>[4x]MNVTVDQSTLAGATRGIVRGGETLKEHRDRLMAATKATGRYAGLKTLELREREPILYNKLFSRLRAGVVDARETAKKIAASPIVEQEGELCFTLYNAAGDSLLTSTGIIIHVGTMGAAIKYMIENNWEANPGVHDKDIFCNNDSLIGNVHPCDIHTIVPIFWEGELIGWVGGVTHVIDTGAVGPGSMATGQVQRFGDGYSITCRKVGANDTLFRDWLHESQRMVRTTRYWMLDERTRIAGCHMIRKLVEEVVAEEGIEAYWKFAYEAVEHGRLGLQARIKAMTIPGTYRQVGFVDVPYAHEDVRVPSDFAKLDTIMHAPCEMTIRRDGTWRLDFEGSSRWGWHTYNAHQVSFTSGIWVMMTQTLIPSEMINDGAAYGTEFRLPKGTWMNPDDRRVAFSYSWHFLVSAWTALWRGLSRSYFGRGYLEEVNAGNANTSNWLQGGGFNQYDEIHAVNSFECAANGTGATAVQDGLSHAAAIWNPEGDMGDMEIWELAEPLVYLGRQIKASSGGSGKYRGGCGFESLRMVWNAKDWTMFFMGNGHISSDWGLMGGYPAASGYRFAAHKTNLKELIASGAEIPLGGDTDPENPTWDAMLPDAQIKRDKQAITTEEMFSDYDLYLNYMRGGPGFGDPLDREPQAVADDINGGYVLERFAGEVYGVVVRKGADGQYGVDETATAAARAQIRKDRLAKSVPVSEWMKGEREKILAKDAGTQVRQMFAASFKLGPRFEKDFRTFWDLPDSWTLPEEEIGVPTYGSRYSMDISELPDVHTVQFVEE;>MNVPVGHLRNVQVLGIDAGGTMTDTFFVDQDGDFVVGKAQSTPQNEALGLIASSEDGLANWGMSLHEALAQLQTGVYSGTAMLNRVVQRKGLKCGLIVNRGMEDFHRMGRAVQSHLGYAYEDRIHLNTHRYDPPLVPRHLTRGVVERTDMMGTQVIPLREDTARDAARDLIAADAEGIVISLLHSYKNPVNERRVRDIVLEEVEKSGKKIPVFASADYYPVRKETHRTNTTILEGYAAEPSRQTLSKISNAFKERGTKFDFRVMATHGGTISWKAKELARTIVSGPIGGVIGAKYLGEVLGYKNIACSDIGGTSFDVALITQGEMTIKNDPDMARLVLSLPLVAMDSVGAGAGSFIRLDPYTRAIKLGPDSAGYRVGVCWKESGIETVTISDCHMVLGYLNPDNFLGGAVKLDRQRSVDAIKAQIADPLGLSVEDAAAGVIELLDSDLRDYLRSMISGKGYSPASFVCFSYGGAGPVHTYGYTEGLGFEDVIVPAWAAGFSAFGCAAADFEYRYDKSLDINMPTETPDTDKEKAAATLQAAWEELTKNVLEEFKLNGYSADQVTLQPGYRMQYRGQLNDLEIESPLAQAHTAADWDQLTDAFNATYGRVYAASARSPELGYSVTGAIMRGMVPIPKPKIPKEPEEGETPPESAKIGTRKFYRKKRWVDAQLYHMESLRPGNRVMGPAVIESDATTFVVPDGFETWLDGHRLFHLREV[4x];>MAYTRSKIVDLVDGKIDPDTLHQMLSTPKDPERFVTYVEILQERMPWDDKIILPLGPKLFIVQQKVSKKWTVRCECGHDFCDWKDNWKLHARVHVRDTPQKMEEIYPRLMAPTPSWQVIREYFCPECGTLHDVEAPTPWYPVIHDFSPDIEGFYQEWLGLPVPERADA[4x]

ACs contain metal ions but not organic cofactors, and use ATP to activate substrates through phosphorylation. The first structural rationale for acetone carboxylation is presented here, focusing on the 360 kDa (αβγ)2 heterohexameric AC from Xanthobacter autotrophicus in the ligand-free, AMP-bound, and acetate coordinated states. Like many carboxylases, AC is a heteromultimeric enzyme complex. Its architecture consists of two heterotrimeric αβγ subunits joined by the interacting α-subunits to form a dimeric core.

To examine the proposed ligand exchange mechanism at the Mn catalytic site, the acetate/AMP-bound structure of AC was characterized. Acetate was used as a product analog because of the instability of the native product acetoacetate in aqueous solution. In this structure, acetate is bound at the Mn site and α-Glu89 resumes its position oriented away from the Mn. The collapse of this channel is apparent in the acetate/AMP-bound structure, which shows a reorganized Mn-proximal α-helix in addition to movement of α-Glu89. Such collapse would prevent the diffusion of intermediates away from the Mn. (d) Our acetate/AMP bound structure describes two intermediates or possibly the acetoacetate product electrostatically displacing Glu89, which results in the formation of the Mn-proximal α-helix. This switch triggers the closing of the interior channel and the reopening of the substrate channel for nucleotide departure and new access.>[6x]MTYSESDIAIVGMNCRYPGVHSVAAFETVLRTGCNILDPKVTPSNGHNHITLNNVYEHMAEFDANFFGYSRAEAEIMDPQQRVFLTCAWEMFEQSGYNPK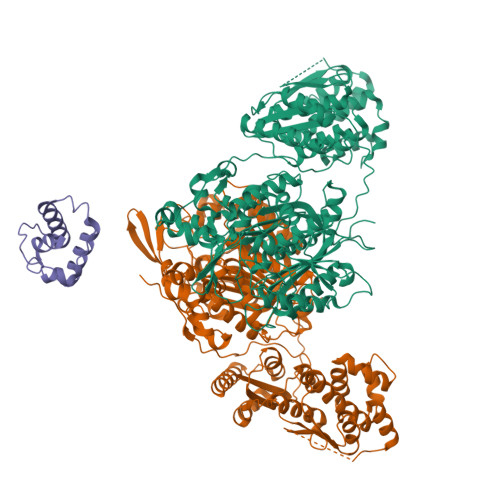QHDARVGLYAGVSTSFYLLTHLMNNPDKLAQLGGLQIMVGNDKDHLTSQLAYRLNITGPCVTVQASCATSLVAVHLACEGLLSGQCDMALAGGVTFRMEEQRSYESHGDGLQAEDGLIHTFDAQASGTVYSSGLGMVLLKRATDAQVQGDNILAVIKGSAINNDGGARSGYTVPGVDGQEAVMIEAHSLAEVTPQQIQYLELHGSGTPLGDAIEFAAIKRVFGTPAPNATPWRLGAVKPNVGHVEMASGITSLIKTVLSLTNRVFYPTLNFQRANPQLGLEDSPFEVVSRLTPWPEGTTPRTAGVSAFGLGGTNAHLVVQAPLSTPQARAQQMGPCVVVLSAKNHNALEQMQNALLAKLAAHPEIRLQDVAYTLRHGRFSAPVRKCVIAENCTQLARQLRDAPMVEATTGCTIYWRLGHRFVVALETLSDWLACSEVLSQAVGQLLEHFPLEPACLQDLSPAQRTFISQYALIALIDERETLNVVLCGDGDGGYAAAVLRGDCTLEQAWHRLNAGQPFDDVPTNPLLQPDVCSLMLDDAASDANRTALEALGQLWLAGVSLDWRWVDAAERMLGSQRIALPGTVFTPQRYWVEAVRPATFSHESSNNLLSRATKSDIIAVVTEIWERTLGVSIDDHHASFFELGGHSLLASTILYDIQQRYGITCTLSAFFADPTIEGLSCYLLEQG~{N}-[(1~{R})-1-[4-(ethanoylsulfamoyl)phenyl]ethyl]-2-methyl-5-phenyl-pyrazole-3-carboxamide | C21 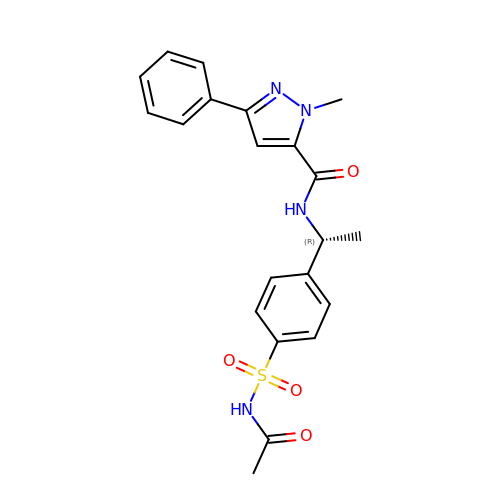H22 N4 O4 S | ALORMMGXOAQIFS-CQSZACIVSA-N>[2x]MKLKKEKKMAEFTFEIEEHLLTLSENEKGWTKEINRVSFNGAPAKFDIRAW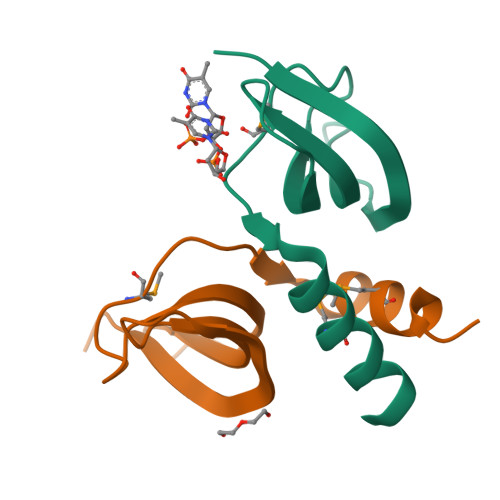SPDHTKMGKGITLSNEEFQTMVDAFKGN>[60x]MAFVDHPPDWLEEVGEGLREFLGLEAGPPKPKPNQQHQDQARGLVLPGYNYLGPGNGLDRGEPVNRADEVAREHDISYNEQLEAGDNPYLKYNHADAEFQEKLADDTSFGGNLGKAVFQAKKRVLEPFGLVEEGAKTAPTGKRIDDHFPKRKKARTEEDSKPSTSSDAEAGPSGSQQLQIPAQPASSLGADTMSAGGGGPLGDNNQGADGVGNASGDWHCDSTWMGDRVVTKSTRTWVLPSYNNHQYREIKSGSVDGSNANAYFGYSTPWGYFDFNRFHSHWSPRDWQRLINNYWGFRPRSLRVKIFNIQVKEVTVQDSTTTIANNLTSTVQVFTDDDYQLPYVVGNGTEGCLPAFPPQVFTLPQYGYATLNRDNTENPTERSSFFCLEYFPSKMLRTGNNFEFTYNFEEVPFHSSFAPSQNLFKLANPLVDQYLYRFVSTNNTGGVQFNKNLAGRYANTYKNWFPGPMGRTQGWNLGSGVNRASVSAFATTNRMEL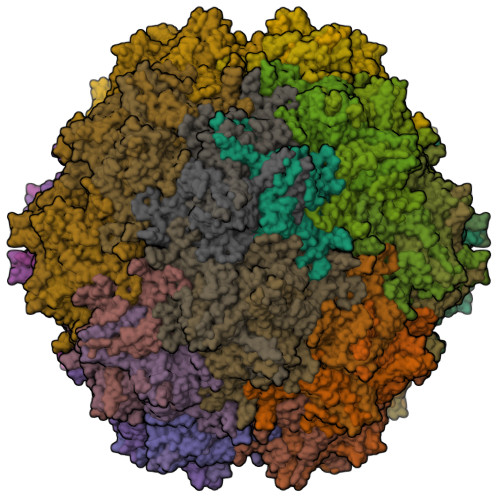EGASYQVPPQPNGMTNNLQGSNTYALENTMIFNSQPANPGTTATYLEGNMLITSESETQPVNRVAYNVGGQMATNNQSSTTAPATGTYNLQEIVPGSVWMERDVYLQGPIWAKIPETGAHFHPSPAMGGFGLKHPPPMMLIKNTPVPGNITSFSDVPVSSFITQYSTGQVTVEMEWELKKENSKRWNPEIQYTNNYNDPQFVDFAPDSTGEYRSTRPIGTRYLTRPL GuxA is a multi-modular and multi-functional enzyme from Acidothermus cellulolyticus whose catalytic domains include a xylanase/endoglucanase GH12 and an exoglucanase GH6, representing a unique combination of these two glycoside hydrolase families in a single CAZyme. GuxA on the other hand contains an N-terminal GH6 domain linked to a CBM3 followed by a GH12 catalytic domain linked to a CBM2 on the C-terminal end. GuxA shows an optimal temperature range between 75 and 80 °C for all three substrates, which is well above the optimal growth temperature of 55 °C for A. cellulolyticus.

The structure of the GuxA GH12 domain was solved with and without cellobiose bound in the active site, to resolutions of 1.5 and 1.85 Å, respectively. The domain exhibits the classic GH12 β-jelly roll, with two curved β-sheets packed together-their concave face forming the active site-and one α-helix. The conserved N-terminal disulfide bridge is present (between Cys7 and Cys38-all residue numberings follow the sequence of the crystal structure), though the electron density indicates that this is partially reduced which might be an artefact of the X-ray diffraction experiment. A second disulfide bridge is also present, in two conformations, between residues Cys73 and Cys78. The active site cavity is lined with aromatic residues that accommodate the substrate without any significant change in structure at the local or whole-protein level—The Cα RMSD between the structures with and without cellobiose bound is 0.166 Å. Glu131 and Glu216 are the catalytic residues (the nucleophile and the general acid/base, respectively), whereas the strictly conserved active site aspartate residue is at position 114. In the case of the A. cellulolyticus GuxA GH12 domain, the leucine at this position probably makes a modest contribution to the enzyme’s thermal stability which, along with the extra disulfide bond, accounts for the thermotolerance of the enzyme. Comparison with the hyperthermotolerant GH12 enzymes suggests that the introduction of several additional salt bridges into the structure could raise the optimum temperature further, which could also be the case for its mesophilic and psychrophilic homologs. Analysis of the protein structure of the GH12 domain of GuxA provides some insight into its increased thermotolerance compared with other GH12 enzymes.

> GTTVTDCTPGPNQNGVTSVQGDEYRVQTNEWNSSAQQCLTINTATGAWTVSTANFSGGTGGAPATYPSIYKGCHWGNCTTKNVGMPIQISQIGSAVTSWSTTQVSSGAYDVAYDIWTNSTPTTTGQPNGTEIMIWLNSRGGVQPFGSQTATGVTVAGHTWNVWQGQQTSWKIISYVLTPGATSISNLDLKAIFADAAARGSLNTSDYLLDVEAGFEIWQGGQGLGSNSFSVSVTSGSAHHHHHH> MGSDKIHHHHHHMKEIDELTIKEYGVDSRILMERAGISVVLA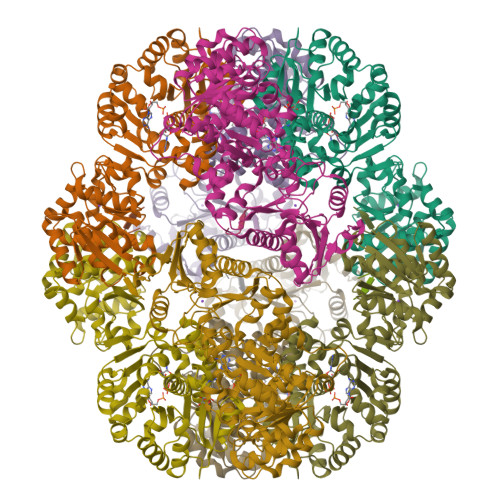MEEELGNLSDYRFLVLCGGGNNGGDGFVVARNLLGVVKDVLVVFLGKKKTPDCEYNYGLYKKFGGKVVEQFEPSILNEFDVVVDAIFGTGLRGEITGEYAEIINLVNKSGKVVVSVDVPSGIDSNTGKVLRTAVKADLTVTFGVPKIGHILFPGRDLTGKLKVANIGHPVHLINSINRYVITREMVRSLLPERPRDSHKGTYGKVLIIAGSRLYSGAPVLSGMGSLKVGTGLVKLAVPFPQNLIATSRFPELISVPIDTEKGFFSLQNLQECLELSKDVDVVAIGPGLGNNEHVREFVNEFLKTLEKPAVIDADAINVLDTSVLKERKSPAVLTPHPGEMARLVKKTVGDVKYNYELAEEFAKENDCVLVLKSATTIVTDGEKTLFNITGNTGLSKGGSGDVLTGMIAGFIAQGLSPLEASTVSVYLHGFAAELFEQDERGLTASELLRLIPEAIRRLKE;> AWLFEA The enzyme IMP dehydrogenase (IMPDH, EC 1.1.1.205) catalyses the oxidative reaction of IMP to xanthosine 5′-monophosphate (XMP), which is subsequently converted to guanosine-5′-monophosphate (GMP) in a reaction catalysed by the enzyme GMP synthase. The reaction catalysed by the IMPDH represents the rate-limiting step in guanine nucleotide biosynthesis and hence IMPDH is an essential enzyme that controls the cellular pool of guanine nucleotides, playing crucial roles in functions such as the immune response or cell proliferation. IMPDH forms tetramers in solution, each monomer consisting of a catalytic and a regulatory domain. The regulatory part, ∼120 amino acids long, is inserted within a loop of the catalytic domain and is composed of two repeats of the cystathionine β-synthase (CBS) domain, constituting a CBS pair or Bateman domain8.

Attempts to crystallize full-length wild-type AgIMPDH in complex with GMP were unsuccessful. However, we obtained crystals of the ΔBateman deletion mutant, in the presence of 10 mM GMP, which diffracted up to 1.25 Å resolution. GMP adopts a conformation identical to that of the substrate, thus confirming a pure competitive inhibition mechanism. Analysis of the enzyme kinetic curves revealed that GMP is a competitive inhibitor with respect to IMP, with Ki=600±100 μM, whereas GDP and GTP do not compete either with IMP or with NAD+, that is, they are mixed-type (allosteric) inhibitors of AgIMPDH, with Ki=210±40 and 160±40 μM, for GDP and GTP, respectively. We further observed that GTP and GDP might bind to the Bateman domain, because the enzymatic activity of a mutant lacking this domain (ΔBateman) was not significantly affected either by GDP or by GTP, in contrast to GMP that inhibited the wild-type and ΔBateman enzymes in a similar manner. ΔBateman and AgIMPDH displayed similar catalytic efficiencies, corroborating previous reports showing that the Bateman domain of IMPDHs is dispensable for catalytic activity. The association of AgIMPDH tetramers change neither the structure nor the accessibility of the substrate to the active site significantly, as the tetramers of ΔBateman-GMP perfectly superimpose over AgIMPDH-GDP.

>GSHMTYRDAATALEHLATYAEKDGLSVEQLMDSKTRGGLTYNDFLVLPGKIDFPSSEVVLSSRLTKKITLNAPFVSSPMDTVTEADMAIHMALLGGIGIIHHNCTAEEQAEMVRRVKKYENGSQDGPLASKSADTKQLLCGAAIGTIDADRQRLAMLVEAGLDVVVLDSSQGNSVFQINMIKWIKETFPDLQVIAGNVVTREQAASLIHAGADGLRIGMGSGSICITQEVMACGRPQGTAVYNVTQFANQFGVPCIADGGVQNIGHITKAIALGASTVMMGGMLAGTTESPGEYFFRDGKRLKTYRGMGSIDAMQKTDVKGNAATSRYFSESDKVLVAQGVTGSVIDKGSIKKYIPYLYNGLQHSCQDIGVRSLVEFREKVDSGSVRFEFRTPSAQLEGGVHNLHSYEKRLFD[2x]>SNARPVWYGEPVDIQPEHRDMMLVVDLSGSMAEEDMKTSNGDFVDRLTAVKQVVSDFIDQRKGDRLGLVLFGDHAYLQTPLTFDRNTVREQLDRTVLNLVGQRTAIGEGLGLATKTFIESNAPQRTIILLSDGANTAGVLEPLEAAQLAKDNHAKIYTVGIGAGEMQVRGFFGKQTVNTARDLDEDTLTKIATMTGGQYFRARNADELAEIYQTIDALEP[2x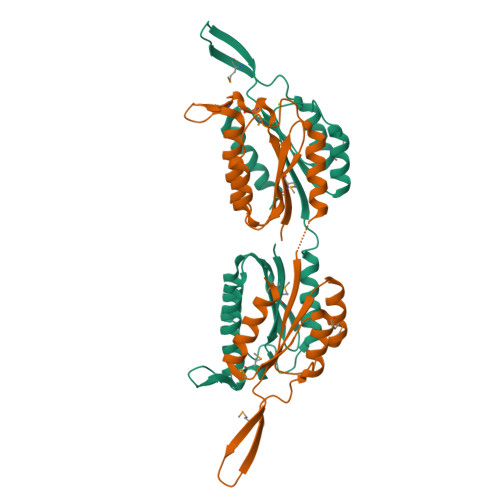]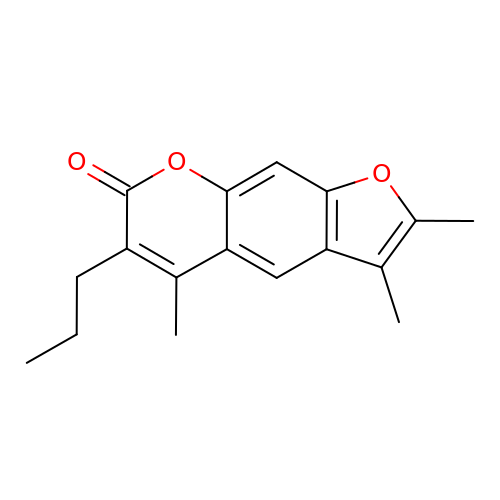2,3,5-trimethyl-6-propyl-7H-furo[3,2-g][1]benzopyran-7-one | C17 H18 O3 | ADGUVFJYVNRVPX-UHFFFAOYSA-N> AAYSQGGGKKKVCYYYDGDIGNYYYGQGHPMKPHRIRMTHNLLLNYGLYRKMEIYRPHKATA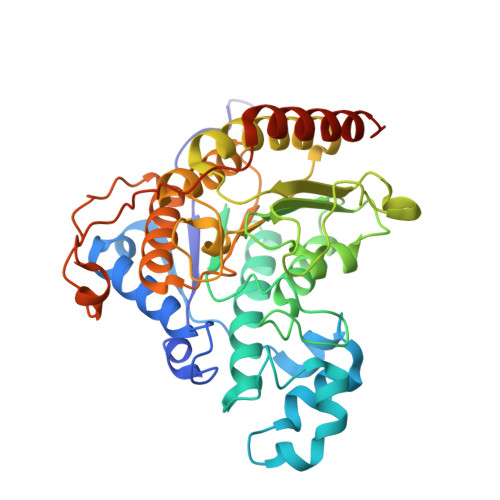EEMTKYHSDEYIKFLRSIRPDNMSEYSKQMQRFNVGEDCPVFDGLFEFCQLSTGGSVAGAVKLNRQQTDMAVNWAGGLHHAKKSEASGFCYVNDIVLAILELLKYHQRVLYIDIDIHHGDGVEEAFYTTDRVMTVSFHKYGEYFPGTGDLRDIGAGKGKYYAVNFPMRDGIDDESYGQIFKPIISKVMEMYQPSAVVLQCGADSLSGDRLGCFNLTVKGHAKCVEVVKTFNLPLLMLGGGGYTIRNVARCWTYETAVALDCEIPNELPYNDYFEYFGPDFKLHISPSNMTNQNTPEYMEKIKQRLFENLRMLPHAPGVQMQAI> MNFLRKIVKNCKDEEIPKPGTPSAPPDDDDLWMPPPEYVPLTQIKGKENVRNFCINGEIKICSPNGYSFRILRHILKSFDNVYSGNRRLIGVVKVVIGLVLSASPVPEGMNWVYKLRRTLIFQWAESHGPLEGEELEYSQEITWDDEAEFVSLQIRVSAKQCHIQGRLWCINMNSKACQLWADMGLKTQQSQ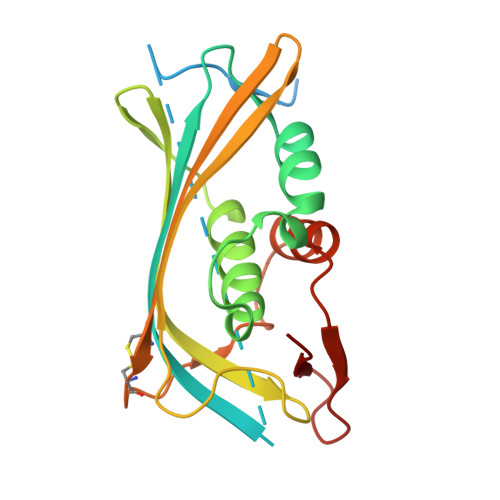EDENTSLLLE>[4x]ASQTITVGSWGG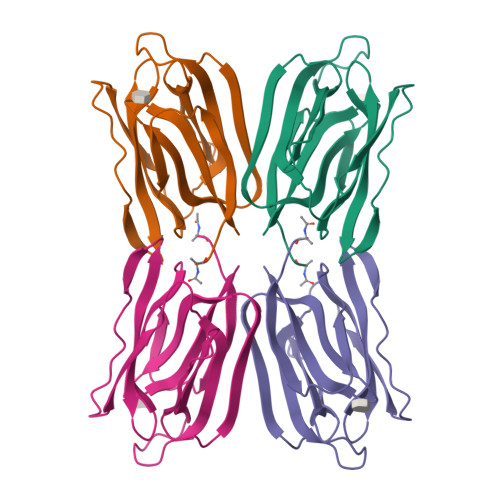PGGNGWDEGSYTGIRQIELSYKEAIGSFSVIYDLNGDPFSGPKHTSKLPYKNVKIELKFPDEFLESVSGYTGPFSALATPTPVVRSLTFKTNKGRTFGPYGDEEGTYFNLPIENGLIVGFKGRTGDLLDAIGIHMSL>[4x]SST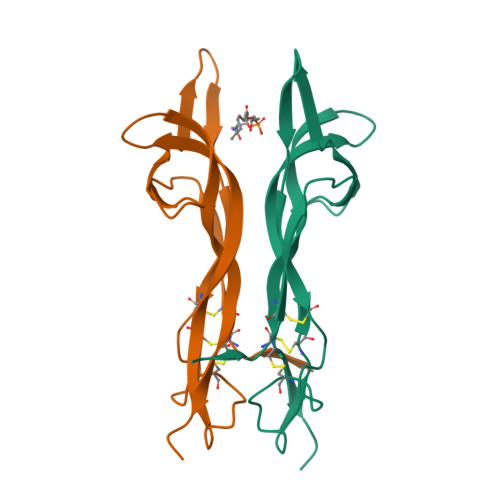HPVFHMGEFSVCDSVSVWVGDKTTATDIKGKEVTVLAEVNINNSVFRQYFFETKCRASNPVESGCRGIDSKHWNSYCTTTHTFVKALTTDEKQAAWRFIRIDTACVCVLSRKATRRG The membrane-anchored SNARE (soluble N-ethylmaleimide-sensitive factor acceptor protein receptor) proteins provide the energy to drive membrane fusion in various cellular contexts, such as intracellular trafficking and exocytosis. Supercomplexes of NSF, α-SNAP, and either a syntaxin tetramer or one of two binary complexes of syntaxin—SNAP-25 reveal atomic details of SNARE processing and show how sequential ATP hydrolysis drives disassembly. NSF comprises three structured domains connected by flexible linkers—the adapter N-domain followed by the D1 and D2 AAA+ domains. Six NSF protomers come together to form the active form of the enzyme, a homo-hexamer.

To improve the resolution of the spire reconstruction, signal subtraction and local alignment were performed as before. This approach improved the reconstruction of the spire proteins to 4.22 Å, enabling docking of a crystal structure of the 2:2 syntaxin—SNAP-25 SN1 complex34 into the density, which was of sufficient quality to assign characteristic side chains, to identify the SNARE domains, and to determine their directionality. Furthermore, we were able to reproduce this result by reconstituting the complex with only the SNARE domains of syntaxin and SNAP-25 under non-hydrolyzing conditions (min22bin20S), yielding the same spire configuration but to a higher resolution of 3.86 Å following local reconstruction. This reconstruction also reveals the interface between an N-domain of NSF and an ɑ-SNAP molecule in detail; the interface is characterized by a core hydrophobic interaction surrounded by charge complementation. Four ɑ-SNAP molecules bind the 2:2 binary SNARE complex, with two SNAP-25 SN1 SNARE domains and two syntaxin H3 domains. Regardless, these structures are consistent with the notion that SNAP-25 SN1 is a critical initial mediator of SNARE assembly.

>SMAEDADMRNELEEMQRRADQLADESLESTRRMLQLVEESKDAGIRTLVMLDEQGEQLERIEEGMDQINKDMKEAEKNLTDLGK[2x];>[2x]MALSEIETRHSEIIKLENSIRELHDMFMDMAMLVESQGEMIDRIEYNVEHAVDYVERAVSDTKKAVKYQSKARRKKIM;>[4x]GMDTSGKQAEAMALLAEAERKVKNSQSFFSGLFGGSSKIEEACEIYARAANMFKMAKNWSAAGNAFCQAAQLHLQLQSKHDAATCFVDAGNAFKKADPQEAINCLMRAIEIYTDMGRFTIAAKHHISIAEIYETELVDVEKAIAHYEQSADYYKGEESNSSANKCLLKVAGYAAQLEQYQKAIDIYEQVGTSAMDSPLLKYSAKDYFFKAALCHFCIDMLNAKLAVQKYEELFPAFSDSRECKLMKKLLEAHEEQNVDSYTESVKEYDSISRLDQWLTTMLLRIKKTIQGDEEDLR;>[2x]GAHMAGRSMQAARCPTDELSLSNCAVVSEKDYQSGQHVIVRTSPNHKYIFTLRTHPSVVPGSVAFSLPQRKWAGLSIGQEIEVALYSFDKAKQCIGTMTIEIDFLQKKNIDSNPYDTDKMAAEFIQQFNNQAFSVGQQLVFSFNDKLFGLLVKDIEAMDPSILKGEPASGKRQKIEVGLVVGNSQVAFEKAENSSLNLIGKAKTKENRQSIINPDWNFEKMGIGGLDKEFSDIFRRAFASRVFPPEIVEQMGCKHVKGILLYGPPGCGKTLLARQIGKMLNAREPKVVNGPEILNKYVGESEANIRKLFADAEEEQRRLGANSGLHIIIFDEIDAICKQRGSMAGSTGVHDTVVNQLLSKIDGVEQLNNILVIGMTNRPDLIDEALLRPGRLEVKMEIGLPDEKGRLQILHIHTARMRGHQLLSADVDIKELAVETKNFSGAELEGLVRAAQSTAMNRHIKASTKVEVDMEKAESLQVTRGDFLASLENDIKPAFGTNQEDYASYIMNGIIKWGDPVTRVLDDGELLVQQTKNSDRTPLVSVLLEGPPHSGKTALAAKIAEESNFPFIKICSPDKMIGFSETAKCQAMKKIFDDAYKSQLSCVVVDDIERLLDYVPIGPRFSNLVLQALLVLLKKAPPQGRKLLIIGTTSRKDVLQEMEMLNAFSTTIHVPNIATGEQLLEALELLGNFKDKERTTIAQQVKGKKVWIGIKKLLMLIEMSLQMDPEYRVRKFLALLREEGASPLDFD> KGIDPFTNPRTVKITASSEETSGENAPASFASDGDMNTFWHSKWSSPAHEGPHHLTLELDNVYEINKVKYAPRQ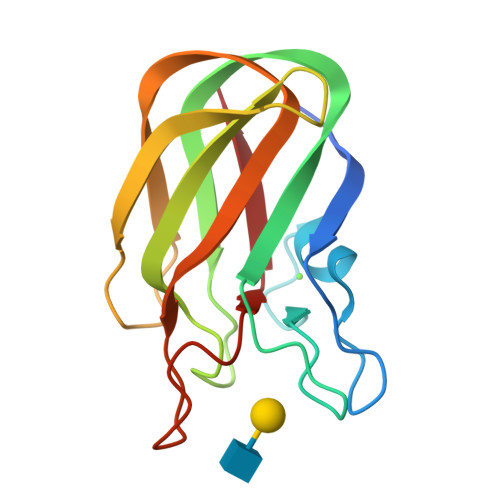DSKNGRITGYKVSVSLDGENFTEVKTGTLEDNAAIKFIEFDSVDAKYVRLDVTDSVSDQANGRGKFATAAEVNVHG> YGPDGDPGDPGDPGPDGKPG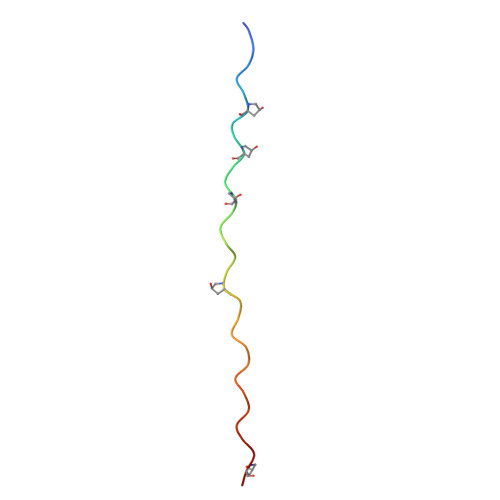PDGPDGPDGDPG> SYDPCTERYSTAYYNRRDVQMALHANVTGAMNYTWATCSDTINTHWHDAPRSMLPIYRELIAAGLRIWVFSGDTDAVVPLTATRYSIGALGLPTTTSWYP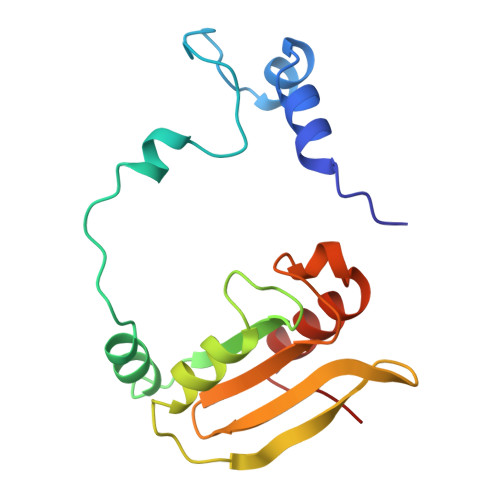WYDDQEVGGWSQVYKGLTLVSVRGAGHEVPLHRPRQALVLFQYFLQGKPMPG>[4x]MLPKATVKRIMKQHTDFNISAEAVDELCNMLEEIIKITTE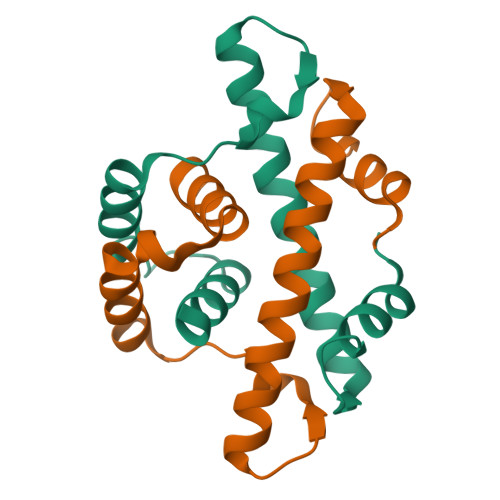VAEQNARKEGRKTIKARDIKQCDDERLKRKIMELSERTDKMPILIKEMLNVITSEL>SDIHELFVPENKLDHVRAEAETLPSLSITKLDLQWVQVLSEGWATPLKGFMREKEYLQVMHFDTLLDDGVINMSIPIVLPVSAEDKTRLEGCSKFVLAHGGRRVAILRDAEFYEHRKEERCSRVWGTTCTKHPHIKMVMESGDWLVGGDLQVLEKIRWNDGLDQYRLTPLELKQKCKEMNADAVFAFQLRNPVHNGHALLMQDTRRRLLERGYKHPVLLLHPLGGWTKDDDVPLDWRMKQHAAVLEEGVLDPKSTIVAIFPSPMLYAGPTEVQWHCRSRMIAGANFYIVGRDPAGMPHPETKKDLYEPTHGGKVLSMAPGLTS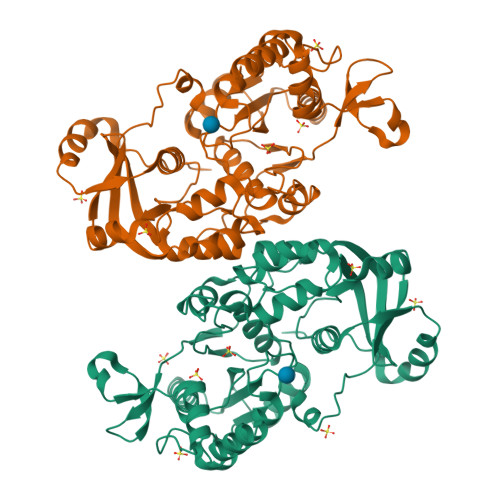VEIIPFRVAAYNKAKKAMDFYDPARHNEFDFISGTRMRKLAREGENPPDGFMAPKAWKVLTDYYRSLEKN[2x]> E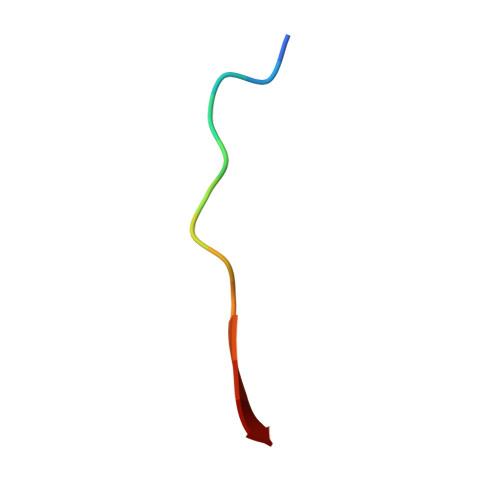RLTLPPSEITLL>HMDTTFQAAIDTGKINGAVVCATDAQGHFVYNKATGERTLLSGEKQPQQLDDVLYLASATKLITTIAALQCVEDGLLSLDGDLSSIAPELAAKYVLTGFTDDESPLDDPPARPITLKMLLTHSSGTSYHFLDPSIAKWRAQYANPENEKPRLVEEMFTYPLSFQPGTGWMYGPGLDWAGRVVERVTGGTLMEFMQKRIFDPLGITDSQFYPVTREDLRARLVDLNPSDPGALGSAVIGGGGEMNLRGRGAFGGHGLFLTGLDFVKILRSLLANDGMLLKPAAVDNMF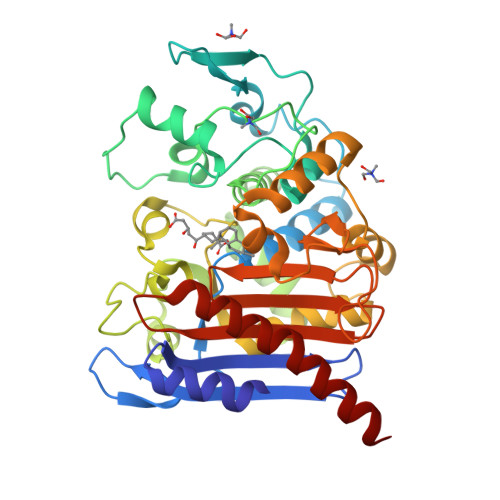QQHLGPEAAASHRAALASPLGPFFRVGTDPETKVGYGLGGLLTLEDVDGWYGERTLTWGGGLTLTWFIDRKNNLCGVGAIQAVLPVDGDLMADLKQTFRHDIYRKYSAWKGQQ[2x]> GPHNMATLTDRTYLPPLEDCLTGRTVILSWRLVASALEDADLARLTSPALSTFLRDGFVHELLKHPARVFEPKDLKQEFETKTSSIQTVAPGVDTIKKDALWLADAVAINQVAALRIVLIEYQTRAHSHLVLPLSTQDVANIQEAAGVGDAHASSILSLLNPASAVDAETMWCDFETEARRRERILATYLSERRSFTAAVDALVTFLLHSAPGQHKDLDSLRRALLKDAFAFDEDLDVPDRSK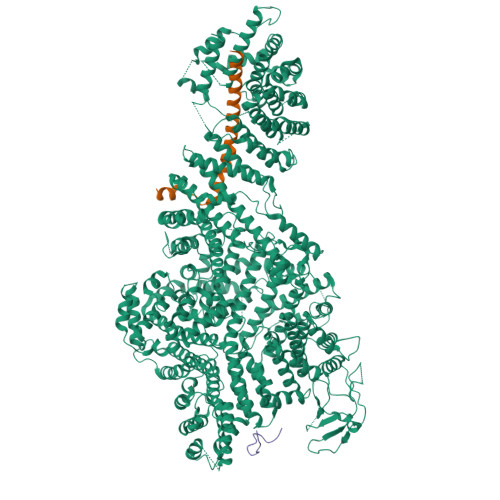LLTMAPTYMNLVEDCIARAQALPAKLGESFKTEAFELDWLRTAITEAVHSLSIAFQALDLDTPYFAPHELLSEWFELMNSSLFLESILGFEVVADLAMPARSLVSAICLKMLNIDRTIQFLHDFDYPDGEEPYLLSSQTLNKIHTAVTNAVNSGVAASLPVAFAWSLIVHQMHLGYQERAERRDLLVNQRAQAGFELEFQPSASTPNRRRRNSAGSIVSLEASPYDDFLREQRLDNDIAPVEQIAMLATSRGQVYQVMSEMALCLGTTHEAAFRPAVGARARLVFQDLLKRSAYLIPYQDEPVFSLLAILATGRQYWDVTDALSASSLNQVYTDMLDDETLFTQFTMQAINRFPYEFNPFSVLCRVLAAALITNKDKADVVTGWLWRTPTLTVDWNPAWDRSYELCFEDENTNSFRLTRDVDLFGSASPARPRHLAAEERFIIPEGTLGRFVTDVGRTARLEFEHSALALLGKRLEVKAAEEICDSGMAPLDVDEQAEAVAMLATVLRAESLKSTAKGGDPEAPLKFLKEASRLLPHNKDILTVISDTIDGLVEKELLELDGPQIAVLASCLQFLHAALAVCPGRVWAYMSRCALIAGDARPGRLSRITGSLDMYAERFDLLSSAVKLFAALIDSAACSAVQRRAGSTALVSVRSAVENPWLGTSEKILSRVALAIAQAALDVYESTTTWRFRSELDRSILVRDVVGLMHKLVVHAHTLSSHLTSTLSPAAAHIISSFLTPPPSASSLRFQPLLGTLLVALITPRATLYPGQSRILAERVTSVLAFCTSLLRAADFLGQTHIPLQTHLFQSACLLARLPAANAVYRAPVLELLRALVEVAGRAANGSGEPPSLLGYLGSHAARSFISLVEGIDKPFGRVEHAVVTWRFFAAVIRNRQQWMAGCLLTGRTPREALKGGGEQKIERKVGEGSVLAAAMERLREVKSLDVQEAVAVMDFVVSAQNYWPWTIFAVRKEKEVVDALRGYVRGLKAPGMVMKTDGAAAAAFQARIAAYVAETFAMQLYHMRQMRQAEKFAGELVADLDYFLREGVMVWGYNASLHGNFARNFAKRFPGVEVDDFKRTMWLPRELGKGYYYALEVAEQMLGFDAGWGGVKQSGFRKEMETANLNLSLVEAQVSLFHAWEYLLLELTLSLLPKKENAAFARQVLQVVEQCLEANQRSQPPENIFVVLGHARAGLALTLLQRLADANQLPRDVTHLLALVSSAIHAVENPFGANDLPYFRTLLKILFVVLRAAKQGTAKPGESNVAITQQVLTILDRVVARCFRALAALVHEQQQNATDGTTTAPEDLALITAILQACLSVPGIEQCQVQVLNIMAAHDVFQVAVALFSWADRLLPANPSPASSSTSTSATNPASGDPVYGELALLFLLELSALPALAEHLACDGLLGHLAAARLAGYMRRTNVGPFAENAGAARCYAIWAKCLLPLLLNILAALGSTVAPEVAWVLNQFPNLLQSSVERIEPPGFSRPTLSLASTPPRQKFISLLEISEIHSLALLTRVLAACRAQNARDVPEVTWDGAKVLECVEYWLRGRKVLRERLVPLGPREVEWRGMVATGGVVGVAGDGGEGCENRLEEKAVGLLVGVREVLEGGLEGEGE;> SGTGLGEVDVDTYLSNLQTKTTLSMIADGLERSARDFDAFLEENVTLEWEAQRKRIYQHFGIK;> SNASRLVTTPQKRAYGFSFSAYGSPTSPSSSASSTPGAFGQSILSSSINRGLNKSISASNLRRSLNVEDSILQPGAFSANSSMRLLGGPGSHKK>[3x]MTTTRTERNFAGIGDVRIVYDVWTPDTAPQAVVVLAHGLGEHARRYDHVAQRLGAAGLVTYALDHRGHGRSGGKRVLVRDISEYTADFDTLVGIATREYPGCKRIVLGHSMGGGIVFAYGVERPDNYDLMVLSAPAVAAQDLVSPVVAVAAKLLGVVVPGLPVQELDFTAISRDPEVVQAYNTDPLVHHGRVPAGIGRALLQVGETMPRRAPALTAPLLVLHGTDDRLIPIEGSRRLVECVGSADVQLKEYPGLYHEVFNEPERNQVLDDVVAWLTERL

Monoacylglycerol lipases (MGLs) resemble a major enzyme class involved in the hydrolysis of monoacylglycerols (MGs) to glycerol and FAs from intracellular and extracellular sources. Due to the increasing prevalence of multi-drug resistant Mtb strains, there is urgent need for the development of new drugs against tuberculosis. mtbMGL emerged as a new promising drug target due to its activity during the dormant and active stage, the reported role in host lipid degradation, membrane synthesis, and the observed severely changed phenotypical appearance of the mtbMGL ortholog in M. smegmatis. mtbMGL harbors an α/β hydrolase core consisting of 8 β-strands surrounded by 6 α-helices (Met1-Val137 and Ala194-Leu279) and a cap region (Ala138-Pro193) containing 3 α-helices. Residues Ser110, His256 and Asp226 form the active site in the core domain of mtbMGL.

The crystals of mtbMGL diffracted to a resolution of 1.8 Å. The cap-region has a Z like shape which resembles the specific architecture observed in other structurally characterized MGLs. The backbone nitrogen atoms of Met111 and Leu39 form the oxyanion hole that can stabilize the transition state intermediate during the catalytic reaction. The catalytic center is located in an approx. 18 Å deep cavity and can be reached from the outside in the observed open conformation via entry between the first and second stretch of the cap region (residues Ala138 to Arg173). The nature of the substrate-binding cavity is governed by predominantly hydrophobic side-chains located in the cap and core domains: Leu39, Ala136, Val137, Ala138, Ala139, Leu142, Val143, Val147, Ala148, Ala15, Leu154, Leu160, Val163, Phe168, Ile171, Val192, Ala194, Leu200, Leu201, Leu228 and Ile229, Pro230. The here presented crystal structure of mtbMGL corresponds to an open conformation in all three molecules of the asymmetric unit and enables a direct access path of the substrate to the catalytic sites. Based on the structural similarities of hMGL and mtbMGL it can be hypothesized that conformational changes in mtbMGL are also realized by a rolling movement of cap helix 1 similar to the one observed in hMGL. No comparable exit hole was observed in any of the molecules of the mtbMGL structure reported here. The mtbMGL crystal structure indicates a monomeric form of the lipase as analyzed with the PISA server, which is in agreement with the size exclusion chromatography of mtbMGL in solution.>AETVSFNFNSFSEGNPAINFQGDVTVLSNGNIQLTNLNKVNSVGRVLYAMPVRIWSSATGNVASFLTSFSFEMKDIK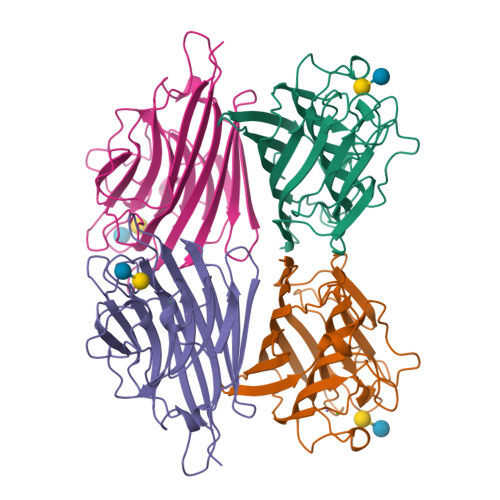DYDPADGIIFFIAPEDTQIPAGSIGGGTLGVSDTKGAGHFVGVEFDTYSNSEYNDPPTDHVGIDVNSVDSVKTVPWNSVSGAVVKVTVIYDSSTKTLSVAVTNDNGDITTIAQVVDLKAKLPERVKFGFSASGSLGGRQIHLIRSWSFTSTLITT[4x]>GDDVKSAC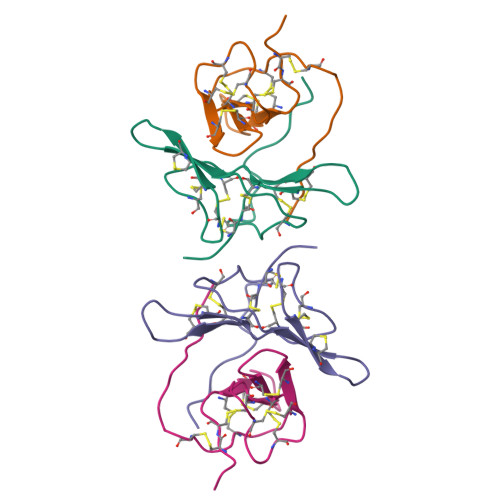CDTCLCTKSNPPTCRCVDVGETCHSACLSCICAYSNPPKCQCFDTQKFCYKQCHNSELEEVIKN[2x]> ISYSDGDQCASSPCQNGGSCKDQLQSYICFCLPAFEGRNCETHKDDQLICVNENGGCEQYCSDHTGTKRSCRCH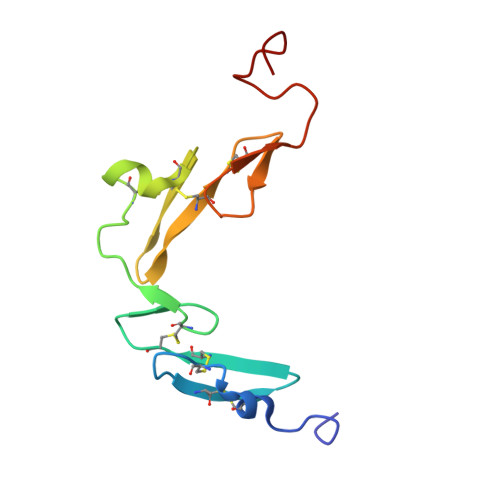EGYSLLADGVSCTPTVEYPCGKIPILE> MKLLEGKRIIVTGGAQGIGASVVRAYIAAGATVASMDMNDTLGQQVV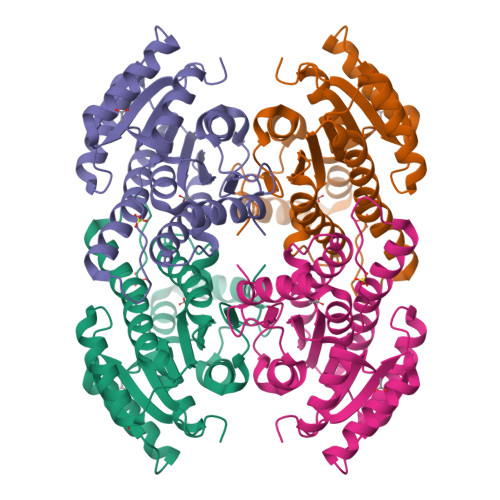SEAGKANPGCKSRYYHCNIADRPEVEKAFATAAEDMGGLDVMVNVAGVHRHSPPDAIAEELYDMLFRVNVLGTINTNAVAYRLMKGQGIGNIINFGSESGLTGEINNALYSATKAAVHTWTRNVARQWGPDGIRINAVLPYMVTPMYVDFRNALSSEDLAAHDAATKTDIPLGGKFGDADKDLAPVMVFLASDASHFMTGQMFPVDGGLIAVR During our attempts to crystallize various oligomeric forms of the cysteine protease inhibitor human stefin B, which is used as a model protein to study amyloid fibrillation and amyloid-membrane perforation, several data sets were collected. The stefin B molecules share the cystatin fold, which is similar to that determined in the crystal structure of the complex with papain and which is composed of a five-stranded β-sheet that is packed against an α-helix. Cystatins are wedge molecules that utilize the N-terminus and two binding loops for binding into the active-site cleft of cysteine proteases. Here, we describe the structure solution, refinement and crystal packing of monomeric molecules of stefin B, which was identified as a crystal structure with rotational order–disorder packing.

The crystal structure of stefin B in space group I4 demonstrates that protein crystals can contain a partial rotational order–disorder structure. The lattice of stefin B crystals is composed of five tetramer layers: four well ordered layers which are followed by an additional layer of alternatively placed tetramers. In addition, the positions of the molecules in the additional layer are related by twofold rotational axes which correspond to space group I422; however, these molecules lie on the twofold axis and can only be related in a statistical manner. When the occupancies of alternate positions and overlapping are equal, the crystal lattice indeed fulfills the criteria of space group I422; when these occupancies are not equal, the lattice only fulfills the criteria of space group I4. The crystal lattice is composed of monomers that are packed in tetrameric rings (as also called tetramers) positioned on top of each other along the fourfold crystallographic symmetry axis. In tetramers, the first binding loop, 46-QVVAG-50, packs against the groove that was formed at the side of the next molecule in the ring. The disordered N-termini fill the area in the centre around the fourfold crystal symmetry axis, whereas the residues of the second binding loop (74-PHENKP-79) are positioned on the external surface of the tetramer. Additionally, assembly analysis using PISA indicates that the tetramers are not a biologically relevant assembly. However, one cannot disregard the differences between the occupancies of the same molecules in crystal 1, which were 0.58, 0.42, 0.51 and 0.49 for molecules 0A, 0B, 5A and 5B, respectively. Hence, we can conclude that the observed crystal disorder is not twinning but rotational order–disorder which was produced by random combinations of unit cells with different positions of tetramers 0 and 5 in an otherwise well arranged crystal network.

>[10x]ATQPATAETQHIADQVRSQLEEKENKKFPVFKAVSFKSQVVAGTNYFIKVHVGDEDFVHLRVFQSLPHENKPLTLSNYQTNKAKHDELTYF> MAFAGAAAPLGVKGRSVFAGMRSFIGQRLGRLYDSFYYS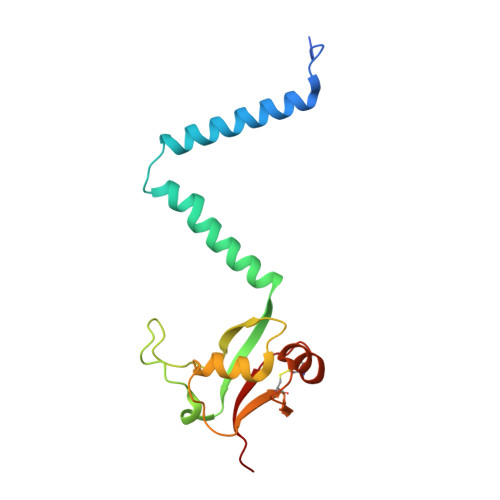QSSTKYVMVFLFPAGIFYTRFRADTKLGYHVFINEEKLYPDYSQNYFDTKWTNGRKVYLDDETTVEQLKAQIYGGKAAPENVKVACRGRVFEDADNVAMAVRAFCKRDPRLLLFQDNL>[4x]MWFGEFGGQYVPETLVGPLKELEKAYKRFKDDE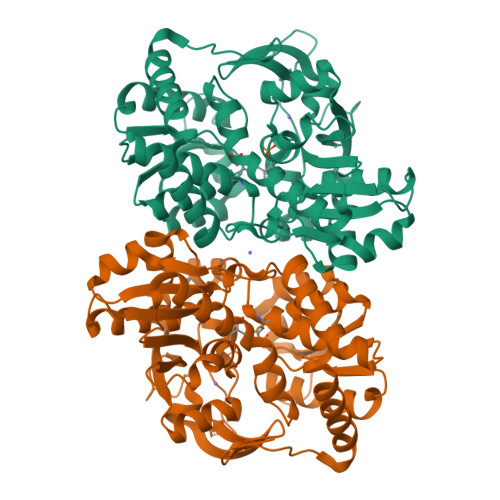EFNRQLNYYLKTWAGRPTPLYYAKRLTEKIGGAKVYLKREDLVHGGAHKTNNAIGQALLAKLMGKTRLIAETGAGQHGVATAMAGALLGMKVDIYMGAEDVERQKMNVFRMKLLGANVIPVNSGSRTLKDAINEALRDWVATFEYTHYLIGSVVGPHPYPTIVRDFQSVIGREAKAQILEAEGQLPDVIVACVGGGSNAMGIFYPFVNDKKVKLVGVEAGGKGLESGKHSASLNAGQVGVSHGMLSYFLQDEEGQIKPSHSIAPGLDYPGVGPEHAYLKKIQRAEYVAVTDEEALKAFHELSRTEGIIPALESAHAVAYAMKLAKEMSRDEIIIVNLSGRGDKDLDIVLKASGNVLEHHHHHH> KITPNLAEFAFSL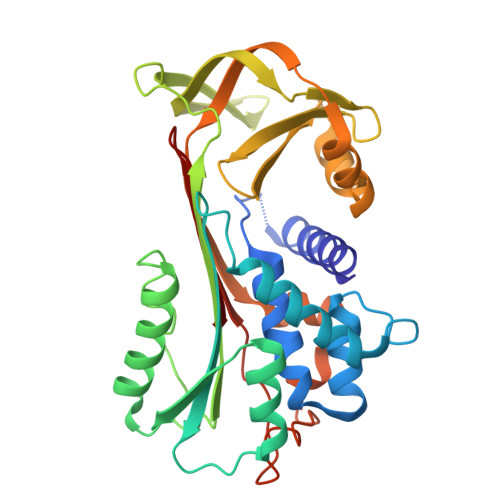YRQLAHQSSTNIFFSPVSIATAFAMLSLGTKADTHDEILEGLNFNLTEIPEAAIHEGFQELLRTLNQPDSQLQLTTGNGLFLSEGLKLVDKFLEDVKKLYHSEAFTVNFGDTEEAKKQINDYVEKGTQGKIVDLVKELDRDTVFALVNYIFFKGKWERPFEVKDTEEEDFHVDQVTTVKVPMMKRLGMFNIQHCKKLSSWVLLMKYLGNATAIFFLPDEGKLQHLENELTHDIITKFLENDRRSASLHLPKLSITGTYDLKSVLGQLGITKVFSNGADLSGVTEEAPLKLSKAVHKAVLTIDEKGTEAAGAMF>[8x]MDLKEFARSQMQAACQYLKEKNPKYDWVGFYVLEHGKLKLEAFVGEKTDHVEINLGDGLCSLAVLKNDIVNEYDVKSNPKYLACFPSTQSEIVVPVRYQGEPIGE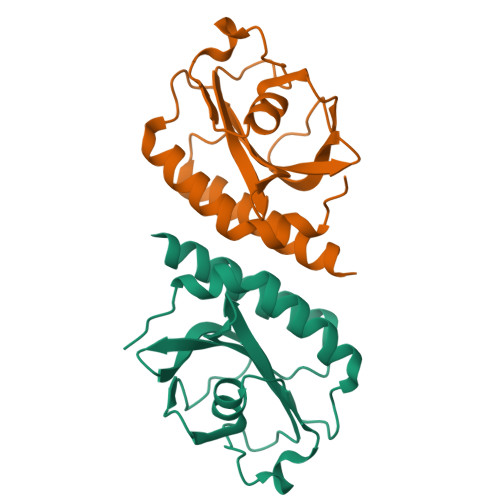IDIDSDKKAAFSKEDEAMLSSIADLMAPLVHEFFVKLEHHHHHH> LGIHSNDTRDAWVNKIAHVNTLEKAAEMLKQFRMDHTTPFRNSYELDNDYLWIEAKLEEKVAVLKARAFNEVDFRHKT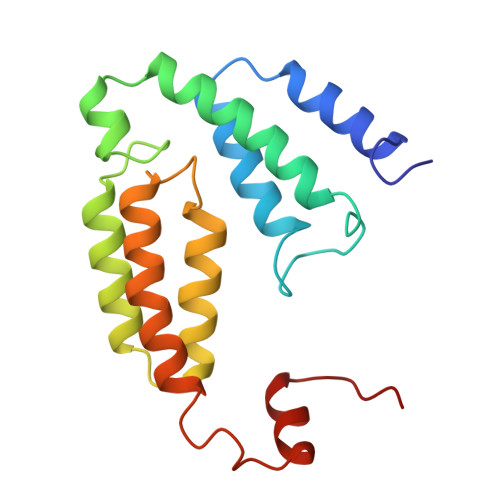AFGEDAKSVLDGTVAKMNAAKDKWEAEKIHIGFRQAYKPPIMPVNYFLDGERQLGTRLMELRNLNYYDTPLEELRKQRGVRVVH> QDDSRYTKFLTQHYDAKPKGRDDRYCESMMVKRKLTSFCKDVNTFIHDTKNNIKAICGKKGSPYGRNLRISKSHFQVTTCTHKGRSPRPPCRYRASKGFRYIIIGCENGWPVHFDESFISP

Angiogenin (Ang, a 14-kDa protein), an unusual member of the superfamily, is a potent inducer of blood vessel formation that was first isolated from the conditioned medium of cultured HT-29 human colon adenocarcinoma cells based solely on its angiogenic activity. The murine Ang family, over the course of evolution, has expanded to accommodate six members: mAng (the murine orthologue of hAng), mAng-2 (also known as mAngRP or mAng-related protein), mAng-3, mAng-4, mAng-5 and mAng-6 27–31. Experiments have shown that mAng, mAng-3 and mAng-4 have angiogenic activities comparable to that of hAng, whereas mAng-2 is not angiogenic 33–35. The main-chain of both mAng-2 and mAng-3 adopts the familiar α/β fold that is characteristic of other Angs and members of the RNase A family.

Interestingly, analysis of the symmetry-related molecules in the mAng-2 crystal structure revealed a two-fold crystallographic dimer that is particularly intimate. The buried surface area at the interface between the two molecules is ∼1100 Å2, consisting of 33 amino acid residues from each molecule with a total of ten ionic interactions across the interface. Interestingly, in the mAng-2 structure, His82, Asp41 and two water molecules from the protomer in the asymmetric unit, along with His113 (an active site residue) from a symmetry-related mate coordinate the Zn2+ ion to complete a penta-coordination. A reciprocal set of interactions makes up the symmetry-related Zn2+ binding site, resulting in a head-to-tail packing. In the mAng-3 structure, the binding site architecture is very similar to that observed for phosphate and sulfate ions in other Ang structures and both anions ligate the same five P1 subsite residues: Gln12, His13, Lys40, His113 and Phe114. However, in the mAng-2 structure, the central sulfate ion interacts with none of the above P1 subsite residues except for the catalytic lysine (Lys40). In mAng-2, the productive conformation is observed for this residue. In mAng-2, Lys40 is expelled and ligates a sulfate ion occupying the active site of a symmetry-related molecule. The mAng-2 structure also reveals Lys40 to be reoriented out of the active site pocket, making it ineffective as a catalytic residue. Although the essential arginine is conserved (as Arg33 in mAng-2 and mAng-3), substitution of Arg31 for Val31 in mAng-2 alters the NLS chemical character. In our structures, however, we observe that mAng-2 has a more open active site than hAng or mAng.>MTTRRLALFDLDHTLLPLDSDYQWADFLARTGRAGDPAEARRRNDDLMERYNRGELTAEQAAEFMLGLLAAHSPVELAAWHEEFMRDVIRPSLTVQAVDVVRGHLAAGDLCALVTATNSFVTAPIARAFGVQHLIATD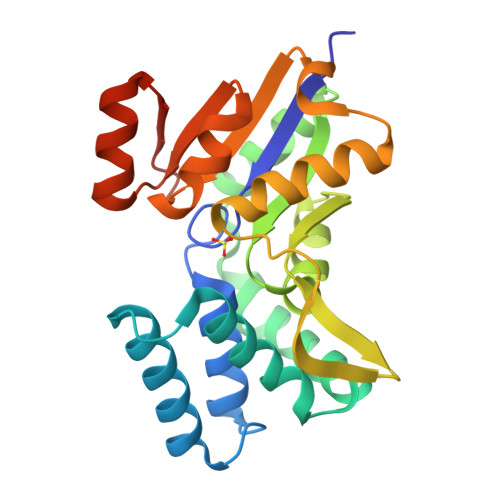PEYRDGRYTGRIEGTPSFREGKVVRVNQWLAGMGLALGDFAESYFYSDSVNDVPLLEAVTRPIAANPSPGLREIAQARGWQVIDLFDHLEDAKS[2x]N'-(5-CHLORO-1,3-BENZODIOXOL-4-YL)-N-(3,4,5- TRIMETHOXYPHENYL)PYRIMIDINE-2,4-DIAMINE | C20 H19 Cl 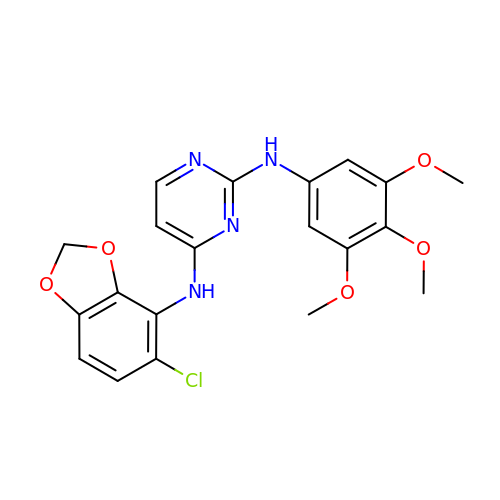N4 O5 | HMKLUOPMOJOUDZ-UHFFFAOYSA-N> GRNAFSELDSADPRVMLRRIIQ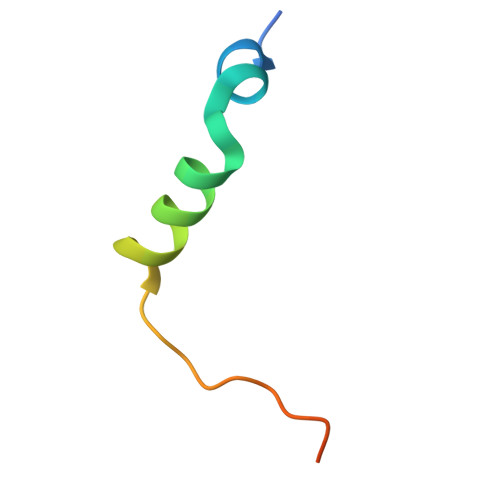NQPQVDPLALQTVQLEP> AKRYWNANLDTYHPKNVSQNRALLTIRVFVHNFNPEEGKGLTFVGSPGVGKTHLAVATLKAIYEKKGIRGYFFDTKDLIFRLKHLMDEGKDTKFLKTVLNSPVLVLDDLGSERLSDWQRELISYIITYRYNNLK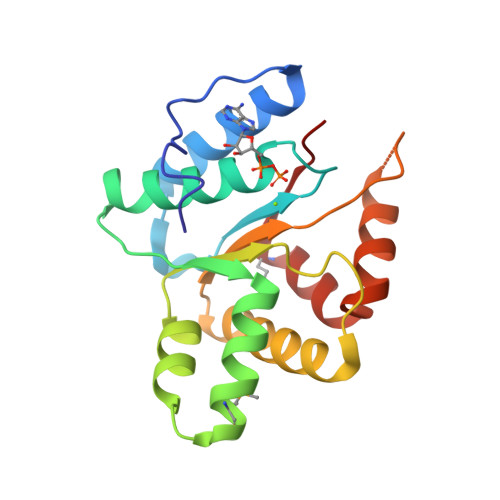STIITTNYSLQREEESSVRISADLASRLGENVVSKIYEMNELLVIK>[2x]MAFRATLSFAGKEFDVLDCTYSLKRDVDSKGRPSSNIYGGQIRLHVESTDDTSILENMTNQ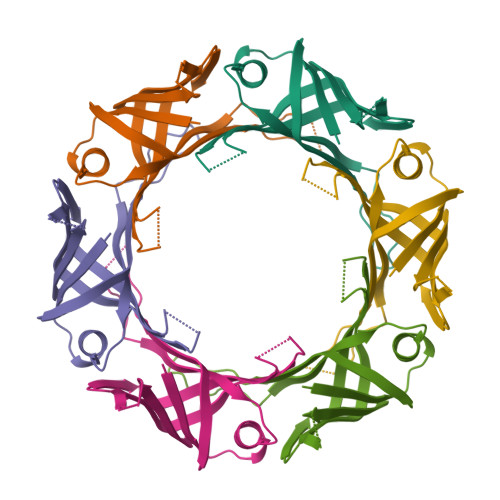FKPHSGSIVFKKGDEEAKMKELTWENGYITEFTENIDIVGSQPMTITFVVSAQVIKIGGAQFEQNWPK> ARTK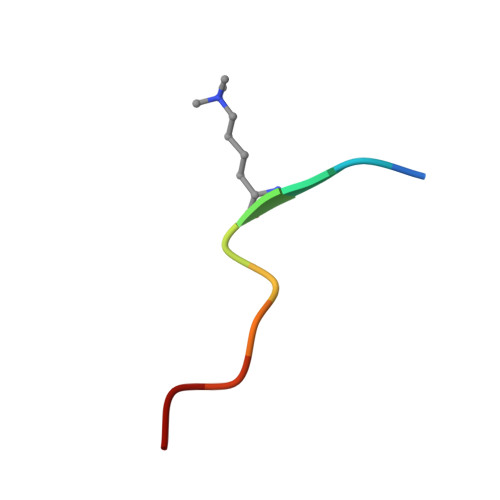QTAAKA>[2x]HHHHHHHEFIPSNTDYPGPHHFEVTFQQSSTAK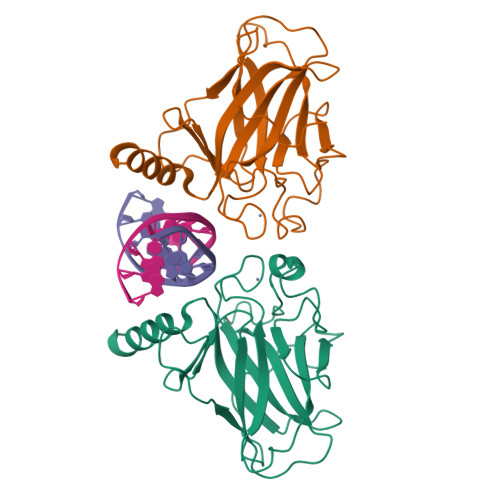SATWTYSPLLKKLYCQIAKTCPIQIKVSTPPPPGTAIRAMPVYKKAEHVTDVVKRCPNHELGRDFNEGQSAPASHLIRVEGNNLSQYVDDPVTGRQSVVVPYEPPQVGTEFTTILYNFMCNSSCVGGMNRRPILIIITLEMRDGQVLGRRSFEGRICACPGRDRKADEDHYREQ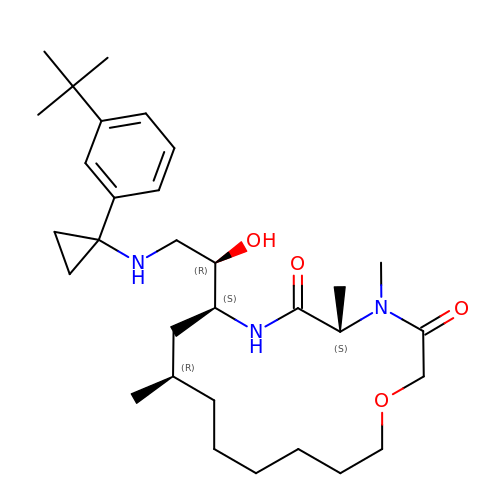(5S,8S,10R)-8-[(1R)-2-{[1-(3-tert-butylphenyl)cyclopropyl]amino}-1-hydroxyethyl]-4,5,10-trimethyl-1-oxa-4,7-diazacyclohexadecane-3,6-dione | C31 H51 N3 O4 | DTTFGMDFRQRNPI-GXVHRJHYSA-N4-[3-(methylsulfonylamino)prop-1-ynyl]-~{N}-[3,3,3-tris(fluoranyl)propyl]benzenesulfonamide | C13 H15 F3 N2 O4 S2 | 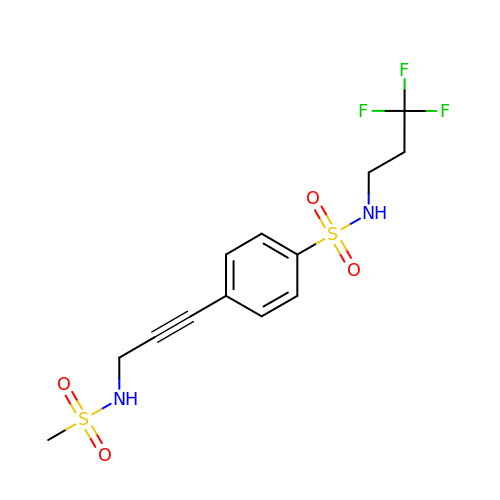KTWYMVDMYCUUFA-UHFFFAOYSA-N>[6x]APVPVTKLVCDGDTYK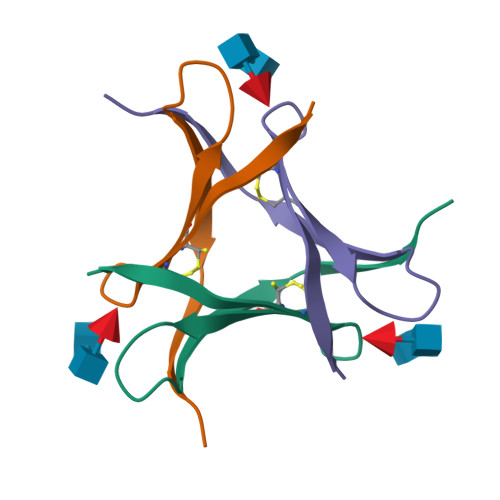CTAYLDYGDGKWVAQWDTAVFHTT(1~{R},3~{S},5~{Z})-4-methylidene-5-[(~{E})-3-[3-(6-methyl-6-oxidanyl-heptyl)phenyl]dec-2-enylidene]cyclohexane-1,3-diol | 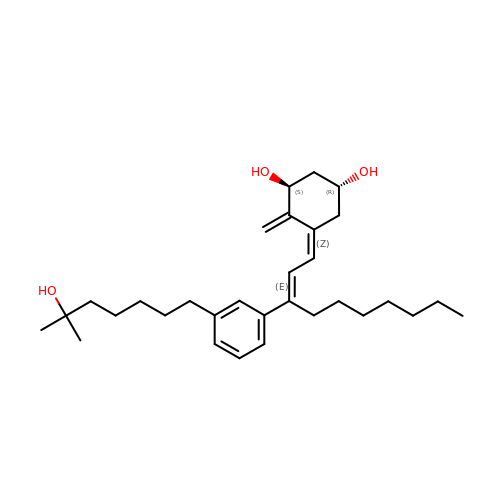C31 H48 O3 | PPRIVUKJJGEEPY-LAWCRIGYSA-N> NSVNPCCDPVICKPRDGEHCISGPCCNNCKFLNSGTICQRARGDGNHDYCTGITTDCPRNRYNV;> NSVNPCCDPQTCKPIEGKHCISGPCCENCYFLRSGTICQRARG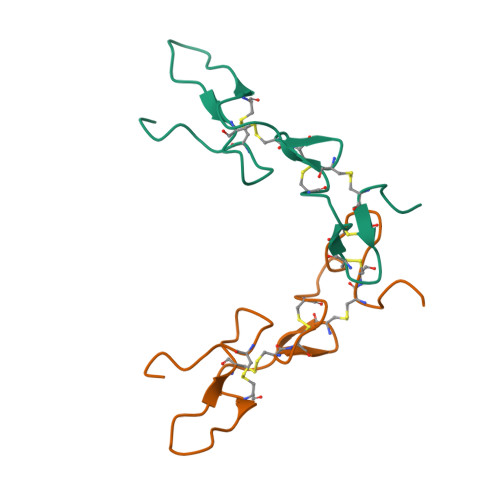DGNNDYCTGITPDCPRNRYNV>SDKIIHLTDDSFDTDVLKADGAILVDFWAEWCGHCKMIAPILDEIADEYQGKLTVAKLNIDQNPGTAPKYGIRGIPTLL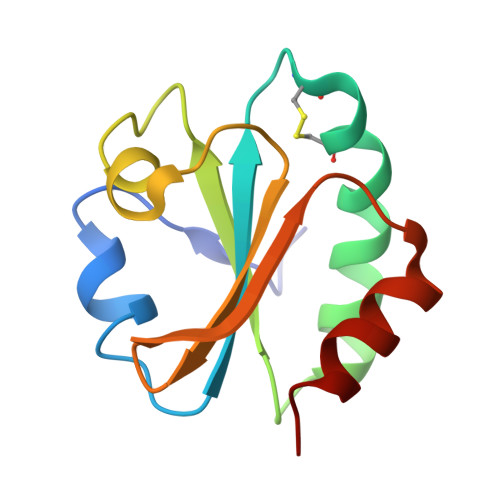LFKNGEVAATKVGALSKGQLKEFLDANLA[2x]>GHMSEKRLPLKPVLRIDFPPGERLGHGKVELMQLIAETGSISAAGRAMDMSYRRAWLLVDALNHMFRQPVICSQRGGKQGGGAALTVFGAELLERYRGMEERMNEALREDIDWLEANRNPQDALNRDREPP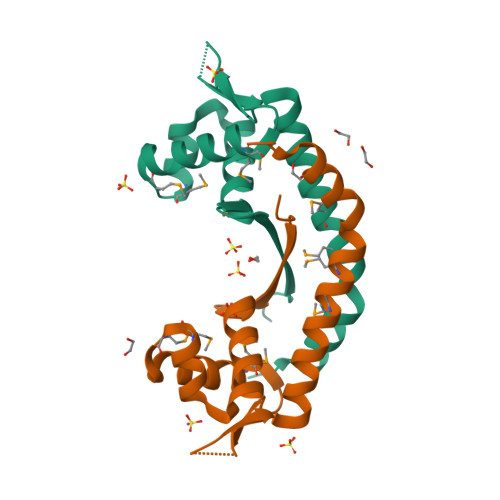TLGS[2x]>[2x]SSESIRMVLIGPPGAGKGTQAPNLQERFHAAHLATGDMLRSQIAKGTQLGLEAKKIMDQGGLVSDDIMVNMIKDE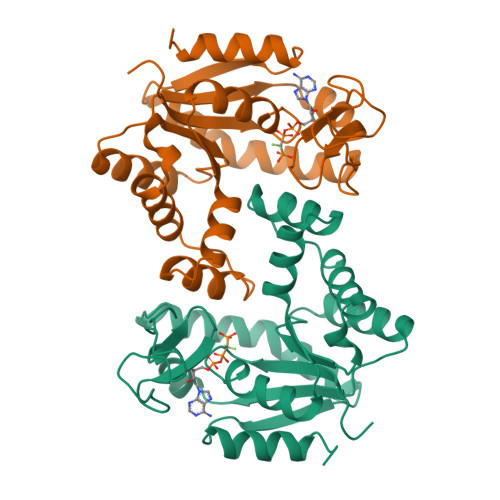LTNNPACKNGFILVGFPRTIPQAEKLDQMLKEQGTPLEKAIELKVDDELLVARITGRLIHPASGRSYHKIFNPPKEDMKDDVTGEALVQISDDNADALKKRLAAYHAQTEPIVDFYKKTGIWAGVDASQPPATVWADILNKLGKN JC96 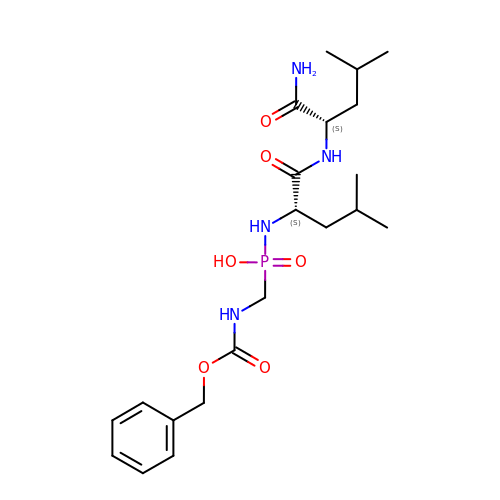| C21 H35 N4 O6 P | DYUJUGYKDAQNDY-ROUUACIJSA-N> 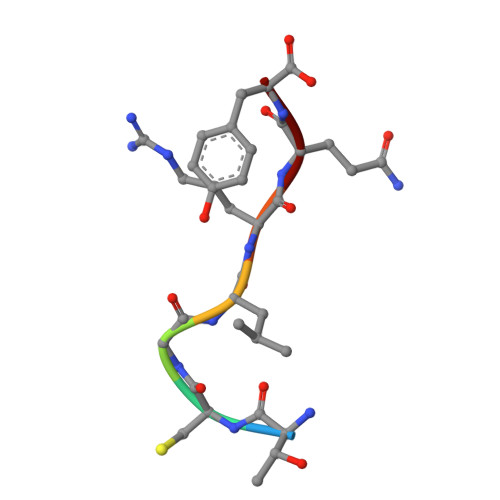TCGLRQY>[2x]MPKEKPHVNIVFIGHVDHGKSTTIGRLLYDTGNIPETIIKKFEEMGEKGKSFKFAWVMDRLKEERERGITIDVAHTKFETPHRYITIIDAPGHRDFVKNMITGASQADAAVLVVAATDGVMPQTKEHAFLARTLGIKHIIVTINKMDMVNYDQKVFEKVKAQVEKLLKTLGYKDFPVIPTSAWNGDN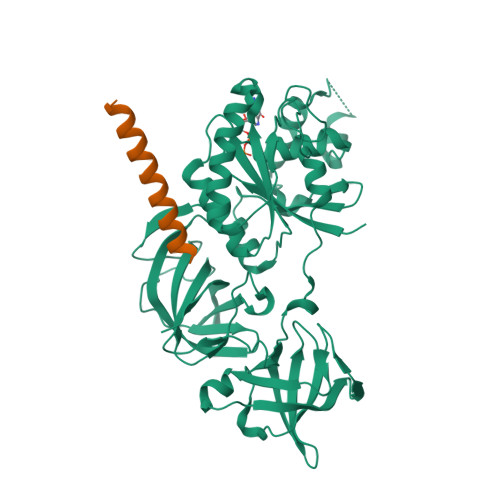VVKKSDKMPWYNGPTLIEALDQIPEPEKPIDKPLRIPIQDVYSIKGVGTVPVGRVETGKLKVGDVVIFEPASTIFHKPIQGEVKSIEMHHEPLQEALPGDNIGFNVRGVSKNDIKRGDVAGHTDKPPTVVRTKDTFKAQIIVLNHPTAITVGYSPVLHAHTAQIPVRFEQILAKVDPRTGNIVEENPQFIKTGDSAIVVLRPMKPVVLEPVKEIPQLGRFAIRDMGMTIAAGMVISIQKGEHHHHHH;>[2x]EEKKEEEKKEEEEKEEEVSEEEALAGLSALFG>MGSSHHHHHHSSGLMDSLLGCGVSAAAREPVPRYLTSQPRVSEVAMQSAPLEQPAKRPRCDGSPRTPPSTPPATANLSADDDFQNTDLRTWEPEDVCSFLENRGFREKKVLDIFRDNKIAGSFLPFLDEDRLEDLGVSSLEERKKMIECIQQLSQSRIDLMKVFNDPIHGHIEFHPLLIRIIDTPQFQRLRYIKQLGGGYYVFPGASHNRFEHSLGVGYLAGCLVRALAEKQPELQISERDILCVQIAGLCHDLGHGPFSHMFDGRFIPRARPEKKWKHEQGSIEMFEHLVNSNELKLVMKNYGLVPEEDITFIKEQIMGPPITPVK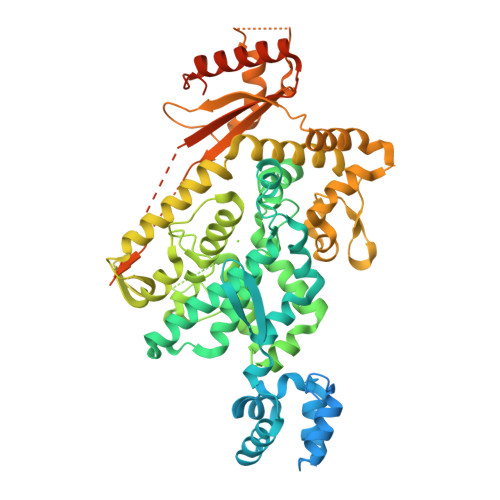DSLWPYKGRPATKSFLYEIVSNKRNGIDVDKWDYFARDCHHLGIQNNFDYKRFIKFARICEVEYKVKEDKTYIRKVKHICSREKEVGNLYDMFHTRNCLHRRAYQHKISNLIDIMITDAFLKADPYVEITGTAGKKFRISTAIDDMEAFTKLTDNIFLEVLHSTDPQLSEAQSILRNIECRNLYKYLGETQPKREKIRKEEYERLPQEVAKAKPEKAPDVELKAEDFIVDVINVDYGMEDKNPIDRVHFYCKSNSKQAVRINKEQVSQLLPEKFAEQLIRVYCKKKDGKSLDAAGKHFVQWCALRDFTKPQDGDIIAPLITPLKWNNKTSSCLQEVSKVKTCLKF[4x]> SNAMLTFYE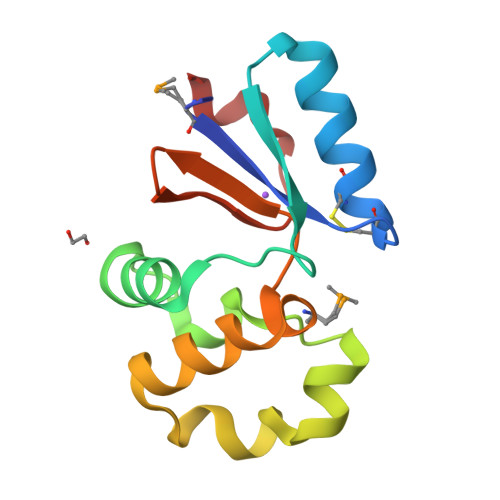YPKCSTCRRAKAELDDLAWDYDAIDIKKNPPAASLIRNWLENSGLELKKFFNTSGQSYRALGLKDKLHQLSLDEAANLLASDGMLIKRPLLVKEGKIVQIGYRTAYEDLDF Herein we report unprecedented location‐dependent, size‐selective binding to designed lanthanide (Ln3+) sites within miniature protein coiled coil scaffolds. [7f] Our design (MB1‐2) features an asparagine (Asn, N), aspartate (Asp, D) hard oxygen donor binding site within the hydrophobic core of a parallel three‐stranded coiled coil (Asn‐Xxx3‐Asp)3, and was found to bind Tb3+, Ce3+, Nd3+, Eu3+, Dy3+, Er3+ and Yb3+, in addition to Gd3+. The structural constraints of binding sites buried within a three‐stranded coiled coil are such that an optimal Ln3+ radius for binding falls between that of Nd3+ and Tb3+. In conclusion, we demonstrate for the first time that designed coiled coils can discriminate between Ln3+ ions based on their size, and that this ability to discriminate is related to the location at which the binding‐site has been introduced.

To elucidate the structural origin of Ln3+ selectivity, a crystal structure of an optimally sized Tb3+ bound to the designed (Asn‐Xxx3‐Asp)3 site in the size‐selective central binding location was obtained. Attempts to crystallise the MB coiled coils repeatedly proved unsuccessful, so an analogous coiled coil scaffold more amenable to crystallisation was adopted, based on CoilSer (CS) and the longer derivative GRAND‐CS, designed by DeGrado and Pecoraro, respectively. The external residues, which are likely critical for the formation of favourable crystal packing interactions, were retained, but the core was replaced with that of MB1‐2. Thus the Leu hydrophobic core of CS was replaced with Ile, and our Asn and Asp binding‐site residues were introduced into positions 12 and 16. The resulting coiled coil, HC02, displays similar Tb3+ binding to that of MB1‐2. To the best of our knowledge this is the first crystal structure of a Ln3+‐binding site engineered within the hydrophobic core of a coiled coil, and provides excellent confirmation of our designed (Asn‐Xxx3‐Asp)3 binding site. The refined structure is consistent with all Tb‐O distances for the binding‐site residues falling between 2.3 and 2.6 Å, in good agreement with previous peptide/protein complexes. Though the electron density cannot assign whether it is the Asn nitrogen or oxygen that is bound, the Tb‐X distances are in better agreement with Tb‐O than the longer Tb‐N distances reported in the literature. With the exception of the terminal residues, involved in the formation of favorable crystal packing interactions facilitated by external Tb3+/Zn2+, all residues, including the binding‐site residues, fall within the preferred region of the Ramachandran plot for α‐helices. Consistent with the experimental evidence of an optimal radius, attempts to obtain suitable crystals with smaller and larger ions, such as Yb3+ and La3+, respectively, have so far been unsuccessful.

>XEWEAIEKKIAANESKDQAIEKKIQAIEKKIEAIEHGX[3x]>MVAPESIVLRVARLDELEQVREILHRIYYPEEGITISYVHGKSHTLDDERFSLSFVEQGTVVVAEDSAAKKFIGVSIAGPIQPGDPDAMVEEAATTETKKWGDILKLLALLERTAD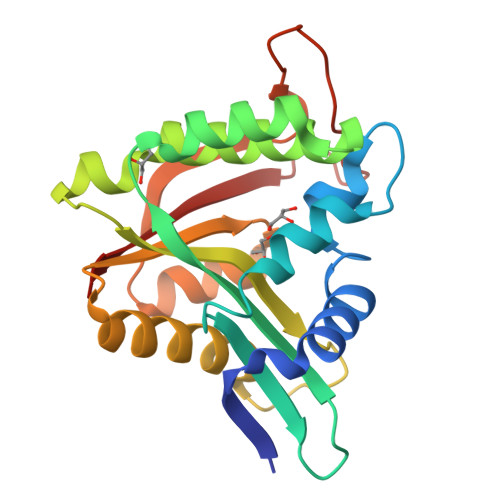VCGRYGLEKAYHVHILAVDPTYRGHSLGQRLLQFQMDLSKKLGFKAISGDFTSVFSVKLAEKLGMECISQLALGDYRDEKGEKLFEPLDVHQVIKTCVKLL[2x]>[2x]WDGKIDGTGTHAMIVTQGVSILENDLSKNEPESVRKNLEILKENMHELQLGSTYPDYDKNAYDLYQDHFWDPDTDNN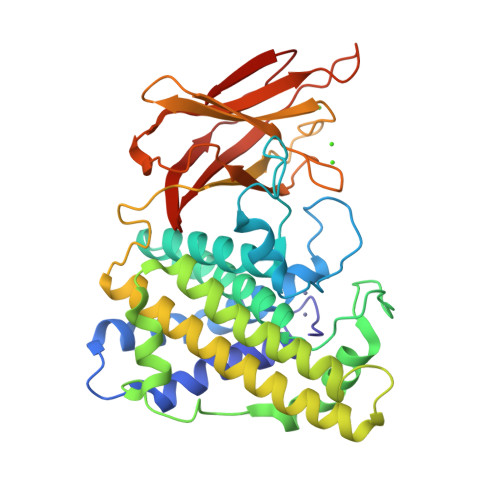FSKDNSWYLAYSIPDTGESQIRKFSALARYEWQRGNYKQATFYLGEAMHYFGDIDTPYHPANVTAVDSAGHVKFETFAEERKEQYKINTAGCKTNEAFYTDILKNKDFNAWSKEYARGFAKTGKSIYYSHASMSHSWDDWDYAAKVTLANSQKGTAGYIYRFLHDVSEGNDPSVGKNVKELVAYISTSGEKDAGTDDYMYFGIKTKDGKTQEWEMDNPGNDFMTGSKDTYTFKLKDENLKIDDIQNMWIRKRKYTAFSDAYKPENIKIIANGKVVVDKDINEWISGNSTYNIK> MAGRWNLEGCTALVTGGSRGIGYGIVEELASLGASVYTCSRNQKELNDCLTQWRSKGFKVEASVCDLSSRSERQELMNTVANHFHGKLNILVNNAGIVIYKEAKDYTVEDYSLIMSINFEAAYHLSVLAHPFLKASERGNVVFISSVSGAL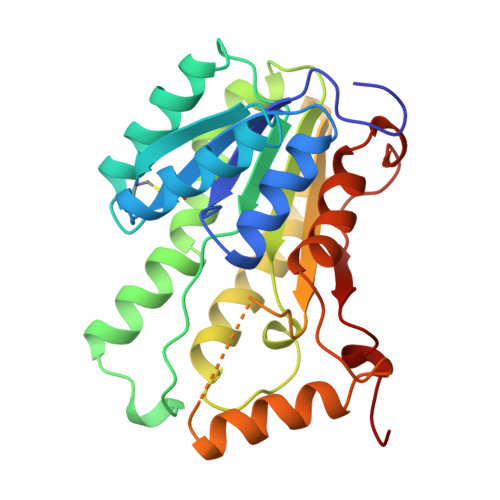AVPYEAVYGATKGAMDQLTRCLAFEWAKDNIRVNGVGPGVIATSLVEMTIQDPEQKENLNKLIDRCALRRMGEPKELAAMVAFLCFPAASYVTGQIIYVDGGLMANCGF> SLASFPVQILPNLYLGSARDSANLESLAKLGIRYILNVTPNLPNFFEKNGD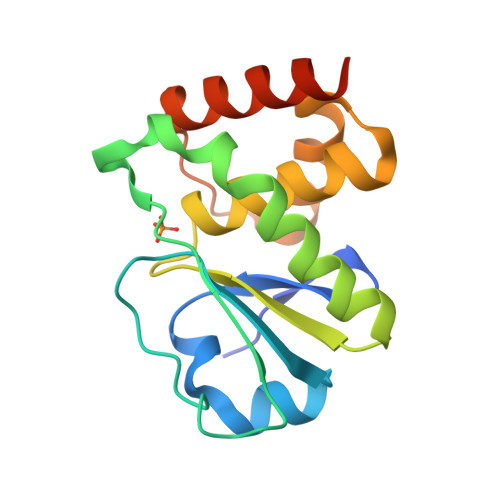FHYKQIPISDHWSQNLSRFFPEAIEFIDEALSQNCGVLVHSLAGVSRSVTVTVAYLMQKLHLSLNDAYDLVKRKKSNISPNFNFMGQLLDFERSLREGHHHHHH>FQNKANVCWAKSLVPILETAGIKLNDRQWSQIIQAFKEDKAYSPEVALNEICTRMYGVDLDSGLFSKPLVSVYYADNHWDNRPGGKMFGFNPEAASILERKYPFTKGKWNINKQICVTTRRIEDFNPTTNIIPANRRLPHSLVAEHRPVKGERMEWLVNKINGHHVLLVSGYNLALPTKRVTWVAPLGV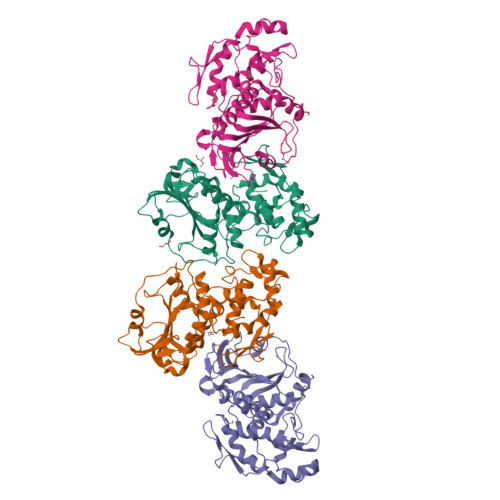RGADYTYNLELGLPATLGRYDLVVINIHTPFRIHHYQQCVDHAMKLQMLGGDSLRLLKPGGSLLIRAYGYADRTSERVICVLGRKFRSSRALKPPCVTSNTEMFFLFSNFDNGRRNFTTHVMNNQLNAAFVG[4x]> MFSSDCEFTKIDCEAKPASTLPAFGFAFNASAPQFASLFTPLLLPSVSPNPNITVPVINDTVSVGDGIRILRAGIYQISYTLTISLDNSPVAPEAGRFFLSLGTPANIIPGSGTAVRSNVIGTGEVDVSSGVILINLNPGDLIRIVPVELIGTVDIRAAALTVAQIS

The exosporium is a prominent bipartite structure comprised of a paracrystalline basal layer and an external hair-like nap. Each filament of the nap is formed solely by a trimer of the collagen-like glycoprotein BclA. One of these proteins is BxpB (also called ExsFA), which is required for the attachment of approximately 98% of the BclA present in the exosporium. In this process, each filament of the nap is attached to a basal layer surface protrusion that appears to be formed by a trimer of BxpB.

To further investigate the nature of the BclA-BxpB attachment, we determined the crystal structure of BxpB. Although it was confirmed by mass spectrometry that the protein used for crystallization contained all 167 residues (data not shown), the structure included only residues 20–167. The crystal structure displayed a trimeric assembly of BxpB monomers. Each monomer folds in a jelly roll-like structure composed of two antiparallel β sheets, labeled A and B, containing six and five strands, respectively. β sheet B includes two β hairpin motifs. A novel feature of the BxpB crystal structure is a bound calcium ion hexa-coordinated by oxygen atoms of residues Asp87, Ser89, Glu94, and Thr153 located on neighboring β turns. The top view of the trimeric structure shows that the β sheets of each monomer form a tight core within the trimeric structure. The crystal structure of BxpB also suggests an orientation for BxpB trimers within the basal layer and a mechanism for BxpB attachment to ExsY. Although the first 19 residues of BxpB are presumably disordered and thus not visible in the crystal structure, the position of residue Thr20 suggests that these disordered residues are most likely positioned at the bottom of the structure shown in Fig. 1B. In either event, the region of BxpB proposed to interface with the BclA NTD is comprised of three loops, two of which are involved in binding Ca2+. Although the crystal structure of the BxpB trimer resembles that of a trimer of the CTD of BclA in several ways, BxpB trimers are much less stable than BclA CTD trimers when treated with heat and detergent. On the other hand, when BxpB trimers are incubated with a peptide containing residues 20–38 of the NTD of BclA, they form a complex with an apparent molecular mass of 55–65 kDa that is as stable to heat and detergent as either BclA CTD trimers or BxpB-BclA complexes extracted from spores.> MEWTREQRYRKYKDWDAQTLLDLQAQAATSPYQMHYHIHPLSGLLNDPNGFSYYNG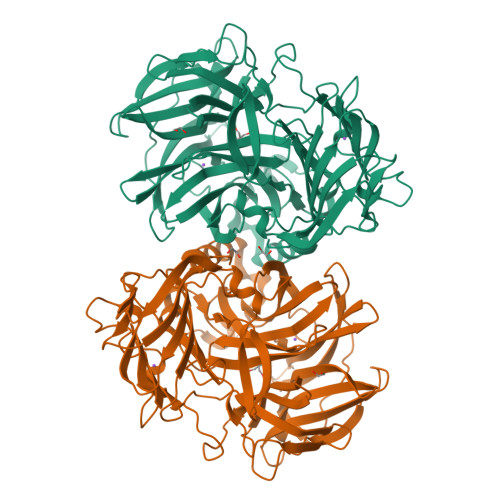EYHLFCQSYPFGPVHGVKSWIHFASPDLVHWHYLGPAIDPDSDLDNAGAYSGSAMEHNGKLLLMYTGNHRDEDWTRIPYQVIAEMDENNHITKPDAAAILPPEHVSEHFRDPQLFKHDGKYYVLLGAQDAETKSGHIDIYESDDLKTWHENGYLDLGKDEMGYMIECPNLVFVNNYPVLIFCPQGLDKAISDYQNIYPNMYWIGKDINLNEAKFTPLQSHPANLDDGFDVYATQAFNAPDGNAYAISWVGLPDCTYPTDKENWANCYSQVKRLEIKDGALYQHPVDAIKNLRHNETQLNDEKIISQKAGKQYELKLYLAAGQAGKLHLASNDDLSASLVIDFNTAQDAKLTIDRASSGPAVNPDYGATRTIGLNDNEDLDLDIFVDGSLCEIFINDGRHVATLRFFARSSNQKIAFDKDTKYTGRLWSMNSIL Pinnatoxin G | C42 H63 N 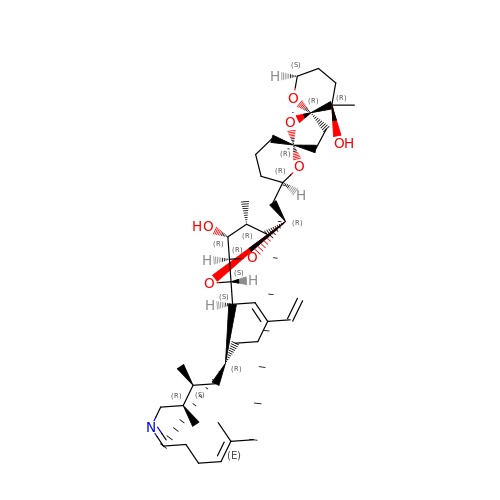O7 | KOWHOZGQQMALMV-WVYVHXBHSA-N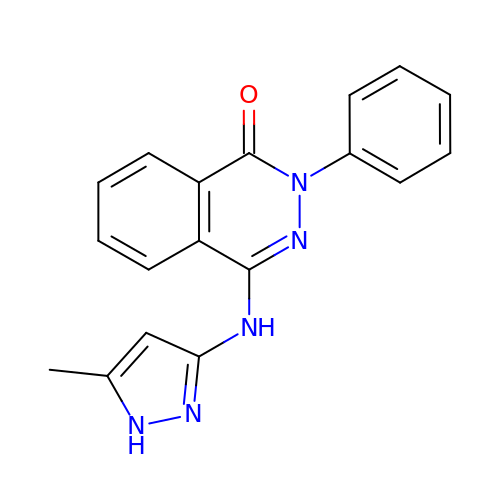4-[(5-methyl-1H-pyrazol-3-yl)amino]-2-phenylphthalazin-1(2H)-one | C18 H15 N5 O | DSDIWWSXOOXFSI-UHFFFAOYSA-N> LISSYNLTQYDT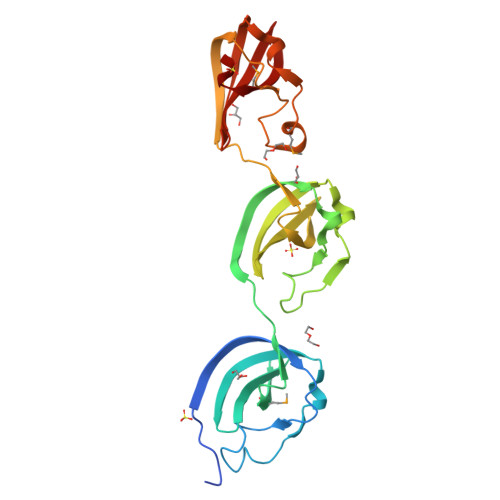LYDTIKQQKNVSEDAKVVKADGHGVYSGIYNTSAASAKKLSTGAPYNNKDVKILKEGTTSRGTWVQFSLNNKVIGWMDKRAFVYYPKATNVKTLNLTGKITAGSTNGLWSEVPGTVNAKKLATTAGAYQNKDAKIIKQGQISGRTYYQFQVGGKTIGWLDARAFHVYDKIQSQSNVNWNRTILNADKHGVYSGVYNTSSSSMNKLSTGAKYNNKKVKVIKQAKTARGTWYQFQVNGKTVGWMDYRAF> ZZHADPICNKPCKTHDDCSGAWFCQACW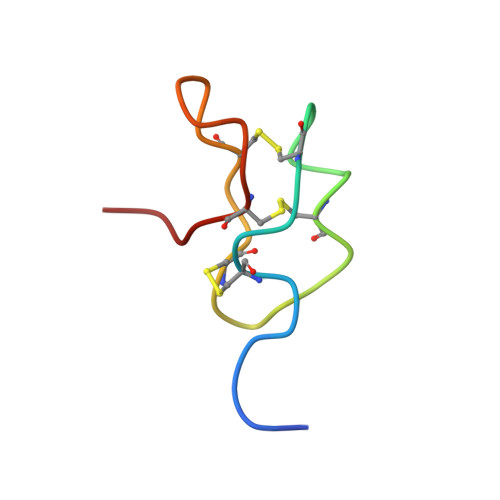NSARTCGPYV>MAYRKRGARRETNLKQDDRMQEKEENKNVNTNSENKNATKPQLSEKVLSQKEEVITDNQEEIKIADEVKKSNKEESKQLLEVLKTKEEHQKEVQYEILQKTIPTFEPKESILKKLEDIKPEQVKKQTKLFRIFEPRQLPVYRANGEKELRNRWYWKLKRDTLPDGDYDVREYFLNLYDQVLTEMPDYLLLKDMAVENKNSRDAGKVVDSETAAICDAIFQDEETEGVVRRFIAEMRQRVQADRNVVNYPSILHPIDHAFNEYFLQHQLVEPLNNDIIFNYIPERIRNDVNYILNMDRNLPSTARYIRPNLLQDRLNLHDNFESLWDTITTSNYILARSVVPDLKELVSTEAQIQKMSQDLQLEALTIQSETQFLTGINSQAANDCFKTLIAAMLSQRTMSLDFVTTNYMSLISGMWLLTVVPNDMFIRESLVACQLAIINTIIYPAFGMQRMHYRNGDPQTPFQIAEQQIQNFQVANWLHFVNNNQFRQVVIDGVLNQVLNDNIRNGHVVNQLMEALMQLSRQQFPTMPVDYKRSIQRGILLLSNRLGQLVDLTRLLAYNYETLMACITMNMQHVQTLTTEKLQLTSVTSLCMLIGNATVIPSPQTLFHYYNVNVNFHSNYNERINDAVAIITAANRLNLYQKKMKSIVEDFLKRLQIFDISRVPDDQMYRLRDRLRLLPVEIRRLDIFNLILMNMEQIERASDKIAQGVIIAYRDMQLERDEMYGYVNIARNLDGFQQINLEELMRTGDYAQITNMLLNNQPVALVGALPFITDSSVISLVAKLDATVFAQIVKLRKVDTLKPILYKINSDSNDFYLVANYDWVPTSTTKVYKQIPQQFDFRASMHMLTSNLTFTVYSDLLAFVSADTVEPINAVAFDNMRIMNEL[10x];> MGKYNLILSEYLSFIYNSQSAVQIPIYYSSNSELENRCIEFHSKCLENSKNGLSLKKLFVEYSDVIENATLLSILSYSYDKYNAVERKLVKYAKGKPLEADLTVNELDYENNKITSELFPTAEEYTDLLMDPAILTSLSSNLNAVMFWLEKHENDVAEKLKIYKRRLDLFTIVASTVNKYGVPRHNAKYRYEYEVMKDKPYYLVTWANSSIEMLMSVFSHEDYLIARELIVLSYSNRSTLAKLVS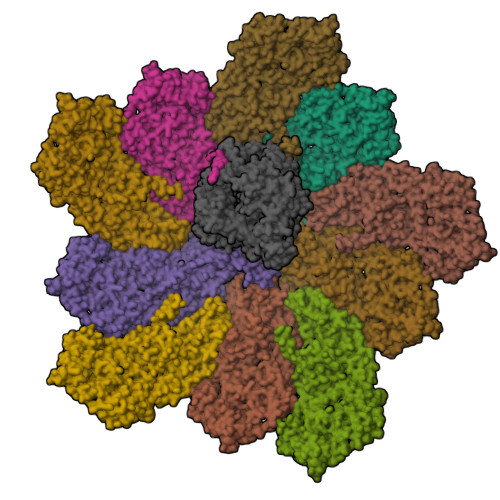SPMSILVALVDINGTFITNEELELEFSNKYVRAIVPDQTFDELKQMLDNMRKAGLTDIPKMIQDWLVDCSIEKFPLMAKIYSWSFHVGFRKQKMLDAALDQLKTEYTEDVDDEMYREYTMLIRDEVVKMLEEPVKHDDHLLQDSELAGLLSMSSASNGESRQLKFGRKTIFSTKKNMHVMDDMANGRYTPGIIPPVNVDKPIPLGRRDVPGRRTRIIFILPYEYFIAQHAVVEKMLIYAKHTREYAEFYSQSNQLLSYGDVTRFLSNNSMVLYTDVSQWDSSQHNTQPFRKGIIMGLDMLANMTNDARVIQTLNLYKQTQINLMDSYVQIPDGNVIKKIQYGAVASGEKQTKAANSIANLALIKTVLSRISNKYSFATKIIRVDGDDNYAVLQFNTEVTKQMVQDVSNDVRETYARMNTKVKALVSTVGIEIAKRYIAGGKIFFRAGINLLNNEKKGQSTQWDQAAVLYSNYIVNRLRGFETDREFILTKIMQMTSVAITGSLRLFPSERVLTTNSTFKVFDSEDFIIEYGTTDDEVYIQRAFMSLSSQKSGIADEIAASSTFKNYVSRLSEQLLFSKNNIVSRGIALTEKAKLNSYAPISLEKRRAQISALLTMLQKPVTFKSSKITINDILRDIKPFFTVNEAHLPIQYQKFMPTLPDNVQYIIQCIGSRTYQIEDDGSKSAISRLISKYSVYKPSIEELYKVISLHENEIQLYLISLGIPKIDADTYVGSKIYSQDKYRILESYVYNLLSINYGCYQLFDFNSPDLEKLIRIPFKGKIPAVTFILHLYAKLEVINHAIKNGSWISLFCNYPKSEMIKLWKKMWNITSLRSPYTNANFFQD>[2x]MKHLEEKTLSTRQIFKGRYLKIEQDQVQAPDGRTYTREYILHPGAAMMIPLLPNGNVVMIHQYRHAVKKVFLEFPAGKRDHNEETLLTAKRELLEETGYEAKDWKFLTTIHPVIGYSNE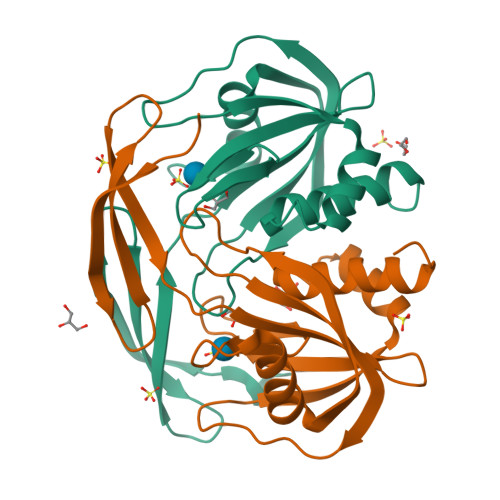HIDLYLARDLTHLEQRLDQGQFIEVVEVKPADLMQLVLEGKVSDVKTQIGAFWLDKFLRGEWN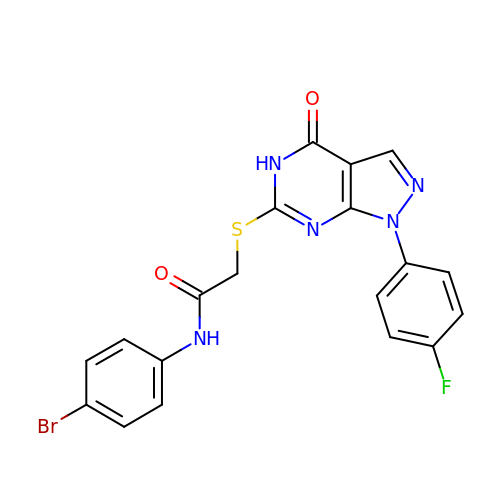N-(4-bromophenyl)-2-{[1-(4-fluorophenyl)-4-oxo-4,5-dihydro-1H-pyrazolo[3,4-d]pyrimidin-6-yl]sulfanyl}acetamide | C19 H13 Br F N5 O2 S | VCFXXKDAPCCCGQ-UHFFFAOYSA-N> MGLFDRLGRVVRANLNDLVSKAEDPEKVLEQAVIDMQEDLVQLRQAVARTIAEEKRTEQRLNQDTQEAKKWEDRAKLALTNGEENLAREALARKKSLTDTAAAYQTQLAQQRTMSENLRRNLAALEAKISEAKTKKNMLQARAKAAKANAELQQTLGGLGTSS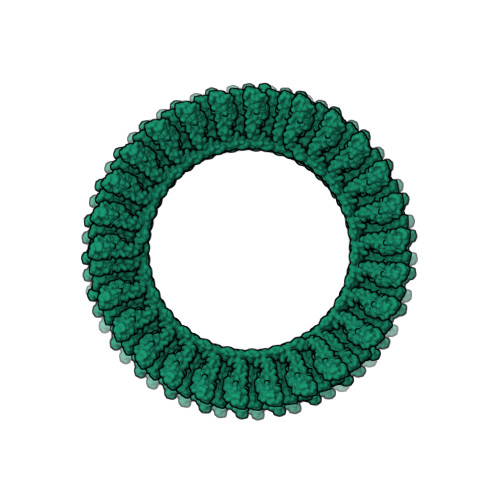ATSAFERMENKVLDMEATSQAAGELAGFGIENQFAQLEASSGVEDELAALKASMAGGALPGTSAATPQLEAAPVDSSVPANNASQDDAVIDQELDDLRRRLNNLAALEVLFQGP> MGNTATEFDGPYVITPISGQSTAYWICDNRLKTTSIEKLQVNRPEHCGDLPETKLSSEIKQIMPDTYLGIKKVVALSDVHGQYDVLLTLLKKQKIIDSDGNWAFGEGHMVMTGDIFDRGHQVNEVLWFMYQLDQQARDAGGMVHLLMGNHEQMVLGGDLRYVHQRYDIATTLINRPYNKLYSADTEIGQWLRSKNTIIKINDVLYMHGGISSEWISRELTL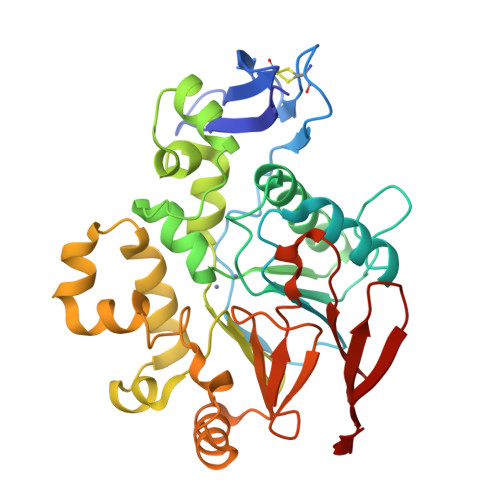DKANALYRANVDASKKSLKADDLLNFLFFGNGPTWYRGYFSETFTEAELDTILQHFNVNHIVVGHTSQERVLGLFHNKVIAVDSSIKVGKSGELLLLENNRLIRGLYDGTRETLQENSLNQ> MSSLQKRPGPGNSSQPTERPRKESILDLSRYQDQRIQATFTGGRQITGILKGFDQLMNLVLDDVEEQLRNPEDGKL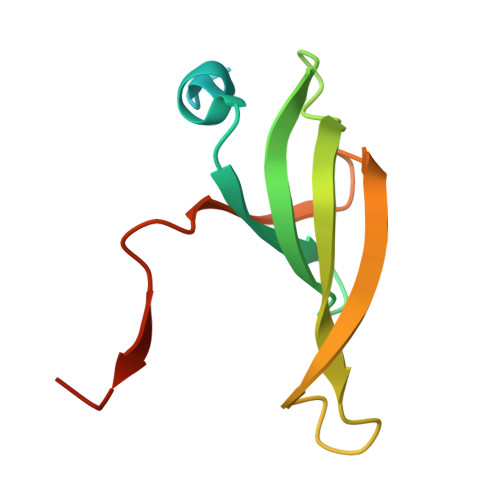TGAIRKLGLVVVRGTTLVLIAPMDGSEEIPNPFVQAE>MRKFILSLSILLSALLVACSSRNHYGDTGSLAGLQAMADSKYTRAQKKQKMGKIREMALKETALSVGAQAGLAWRAKIIDEQLNKQARNLDAIYDFNSLVLEHNILPPVLLEGRNTLNLADAQSIRISDRTYKVAKQAHFITTPPTWRQYLWMDYVKPEAPNVTLLPKTKAEKEIWCIYTERGWKNGIDQANTILEENIARIKEDFGGMILYRKLLAMNMVSPPYVSHTDLGVTGDGSEIHIDDRVLRITALPELNVNSAEWRAAVAKDENALERFKNMEKLANQAKIVITNKSWQPIIAPVS[13x];>MNNNKIVIMFIFSALLAGCAGTMKFKKPPINNPSDDATIKLAEAAVSVSDSMLEMAKVEKVITPPSKDNTLTIPNAYNLQARASVDWSGPIEELTARIAKAAHFRFRVLGKSPSVPVLISISTKDESLAEILRDIDYQAGKKASIHVYPNSQVVELRYAKIYS[26x];>[31x]MMAEHDQNNDEYKFAELDSYDMDQAGESDLDSEASYQSGKEGLTKKKDIKRNALIAIGAVVFIMVMYKIIGWMFFSDKSSQVTSKPAIPPVTQVATPQPVQTIPTTTPIQQVQPTTIIEDDPDLKKKVSAIEMTQQSLRSEVNALSEQINAVNNNIKNLNAQIVNLNQIIGNMSNQIARQSEVINVLMARTTPKKVVKVSRPIVQARIIYYIQAVIPGRAWLIGSNGSTLTVREGSKIPGYGMVKLIDSLQGRILTSSGQVIKFSQEDS;>MASKKENLKSLFSNTRTRVIIIFTAALLIIAVVIGFFKIRGATTGSIAAAEVSTVPGGIQSIPGVLDPTAQYAKLQEEQNITQAQVAEKTGGSAIPTIIRTQALGEGVGVIGSQSGVGFAALAQEELGGPQRSLWIQELQDGSCSKSVITKVVNQGAQLTDLKAACSCVQLKDSGYGLQELEQVCECKELKSAGYNARQLKEAGYSAGRLRNCGFDACELRNAGFTAQEMKDGGFSDGELKGAGFSDAEIAKASGLPDGITADDVRKAGCGAAALAKLRQAGVSASAIRKISGCTAEQLKAAGYTAKELKDAGFSAADLRRAGFSAAELKDAGFTARDLLNAGFTPADLAKAGFSDAQIKAAQAELPPGITPQDVKNAGCDVEALKKEREAGVSAALIRQYAGCSAQALKAAGFTDADLANAGFTPAQISAATPLSDAEIKAAGCDPDKLKKLFSAGVSAKRIKELNGCSAEALKAAGYDAQSLLAAGFTPQELLAAGFTPKQLEDAGLNPVSIIADGRVADCSVESLKKARAAGVSALTIKQTLGCSAAALKAAGYTAKELKDAGFTAAELKAAGFSAKELKDAGFTAKELRDAGFSAQELKDVGFSAKDLKDAGFSAAELKAAGFTAAQLKAAGFSAKDLKDAGFSAAELKAAGFSAKELKDAGFSASDLKNAGFSAKELKDAGFSASDLKSAGFSASELKNAGYSADELKKAGYTSAELRNAGFSPQESAVAGLQGPDLQQLDSSITGIPSIPGATPRPTTSDAASSAEQLQAILQKQNEQLAEQKYQQEIQQRTSDMLTAATQLVQDWKQVETQVYTEGTEETKTSGGESAVPGTGTGTGSNNQPVDQGAVSAQNQAIIKTGDIMFAVLDTSVNSDEPGPILATIVTGKLKGSKLIGSFNLPSNADKMVITFNTMSIPGAEKTISISAYAIDPNTARTALASRTNHHYLMRYGSLFASSFLQGFGNAFQSANTTITIGGTGGGNNITVANGVGRSTLENAVIGLATVGKAWSQQAQQLFNTPTTVEVYSGTGLGILFTQDVTTI[18x];>[18x]MMKKYDQLCKYCLVIGLTFSMSCSIYAADQSDDAQQALQQLRMLQQKLSQNPSPDAQSGAGDGGDNAASDSTQQPNQSGQANAPAANQTATAGGDGQIISQDDAEVIDKKAFKDMTRNLYPLNPEQVVKLKQIYETSEYAKAATPGTPPKPTATSQFVNLSPGSTPPVIRLSQGFVSSLVFLDSTGAPWPIAAYDLGDPSSFNIQWDKTSNTLMIQATKLYNYGNLAVRLRGLNTPVMLTLIPGQKAVDYRVDLRVQGYGPNAKSMPTEEGIPPSANDLLLHVLEGVPPPGSRRLVVSGGDARAWLSNEKMYVRTNLTILSPGWLASMTSADGTHAYEMQKSPVLLVSWHGKVMQLKVEGL;>[13x]MRSLRTNYIYVLFKTTGLLFLLLLSACNRSGYIPENEVPKLPCRVDGACDATIIKMMTDLNKKGIKVASVGQNYLISIPASALFADQSPRLNWASYSLLNEIAAFLKQFRKIAITVTSYSSKYVSVKRERALTLARSRVVSEYLWSQGVDSRIIFTQGLGSDKPITSYTLGGDRSPNARVEITFRRAVA;>MRNLMRCLIMIKSLIKGVDMSRKLAKTRILGYGLMICFLAGCFHPPYNNFQPDRRAVKRVGVDTGIGAVAGAIASGTASGTLIGAAAGGTVGLVASIYRDSKRKIIRDLQKQDIQYVEYGDTRTLIIPTDKYFMFSSPRLNEICYPGLNNVIRLLNFYPQSTIYVAGFTDNVGSRSHKRKLSQAQAETMMTFLWANGIAAKRLKAEGYGDKNAISDNAIIHGSAQNRRIEIQWFTSPAQPPQPQMAYVK[13x];>[13x]MLKRCYLLILLMFVLASCAHHKPQTPPAEVKKQGTSSTRQFRQVSSFNQIVVQGRLNVNLHTGYNKPEVMLRGDPRDLVQVRTIVKQNTLYVSLGQGYPDYGAVTVDIKTKFLNRFRYEGAGVVTGNNLRTSYLDLYLANEGTTRLAGNIGLQKLEAVGNGVTQINGVSSRNLQIVLKGDPKVLISGFVNLRQLDMYGKGTLSLYWIKSDTLTIRAKKAAKIQLAGIVNRLDVELWDFAQFKGKYLRAQRSFVKTHDKSVAEISAVNHQSSLATDASDIYYYNLSKTRADFMAFNGSVLDMREWGQSDLKDFDRYNKQFP;>[13x]MLFLKIKTNQRTTMNILKPKAFLLASVFVLSISPAFAADGCCSKMGGINYCDSSAGRLVCNNGFYSTCYCTRHAVMDLQFLMGCCLWHGGVYPQLNSSGLVVCNDGYVSEECSLQKPVEQISVY

Legionella pneumophila is an opportunistic pathogen that causes the potentially fatal pneumonia known as Legionnaires’ disease. The pathology associated with infection depends on bacterial delivery of effector proteins into the host via the membrane spanning Dot/Icm type IV secretion system (T4SS). The Dot/Icm complex of L. pneumophila is one of the largest known T4SSs. The Dot/Icm T4SS has as many as 300 protein substrates, a striking contrast to the H. pylori Cag and B. pertussis Ptl T4SSs, each of which transports only one virulence factor.

We have determined a 3.8 Å asymmetric reconstruction (C1) of the Dot/Icm T4SS using single particle cryo-EM approaches. This resolution made it possible to trace connections between the OMC, which contains 13 copies of the asymmetric unit, and the PR, which contains 18 copies of the asymmetric unit. Unexpectedly, we observed five peptide chains originating from the PR, with attached densities sandwiched between the PR and OMC. The models that were generated from the 2.8 Å resolution, symmetry-imposed reconstructions of the OMC and PR were fit into the 3.8 Å map of the Dot/Icm T4SS that was generated without the imposition of symmetry. First, we observe 13 linkers between the OMC and PR (identified as residues 264–270 of DotH) in various conformations, revealing the direct connections between the two regions. Second, we observed five small globular folds located between the OMC and PR. These folds consist of two β-sheets and incorporate the linker from DotH as an additional β-strand in one of the two sheets. Close inspection clearly showed that these domains contain folds nearly identical to that of the C-terminal domain of DotH in the OMC (residues 278–360). Thus, there are 18 copies of DotH in the entire structure with all 18 NTDs comprising the PR, 13 of the associated CTDs extending up to build part of the OMC disk, and the other five CTDs extending up only part way into the intervening space. The flexibility of these five DotH CTDs suggests a mechanism through which the symmetry mismatch observed between the OMC and PR can be accommodated though the utility of the symmetry mismatch cannot be inferred.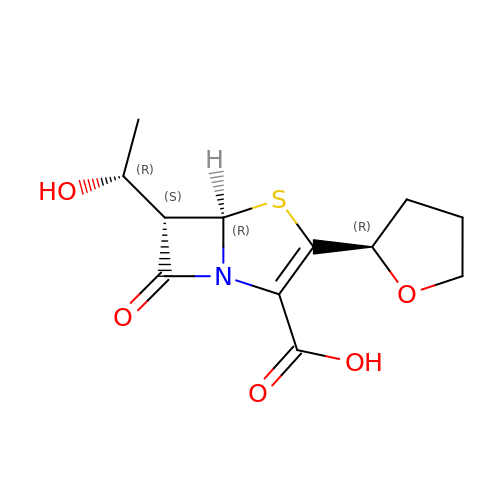(5R,6S)-6-(1-hydroxyethyl)-7-oxo-3-[(2R)-oxolan-2-yl]-4-thia-1-azabicyclo[3.2.0]hept-2-ene-2-carboxylic acid | C12 H15 N O5 S | HGGAKXAHAYOLDJ-FHZUQPTBSA-N> GIDPFTKHGQKECDNALRQ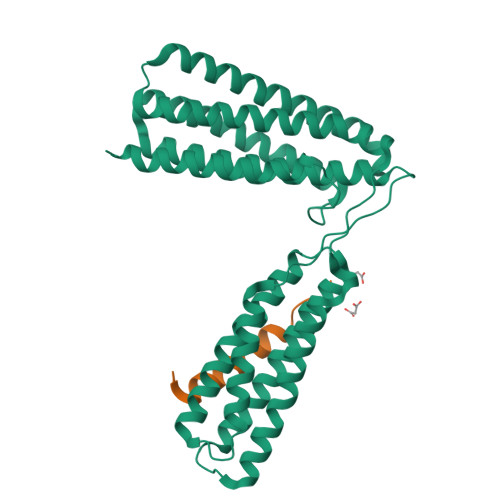LETVRELLENPVQPINDMSYFGCLDSVMENSKVLGEAMTGISQNAKNGNLPEFGDAIATASKALCGFTEAAAQAAYLVGVSDPNSQAGQQGLVEPTQFARANQAIQMACQSLGEPGCTQAQVLSAATIVAKHTSALCNSCRLASARTANPTAKRQFVQSAKEVANSTANLVKTIKALDGDFTEENRAQCRAATAPLLEAVDNLSAFASNPEFSSVPAQISPEGRAAMEPIVISAKTMLESAGGLIQTARALAVNPRDPPRWSVLAGHSRTVSDSIKKLITSMRDKAPGQL;> PELDDILYHVKGMQRIVNQWSEK>MKLSDLISRWIDVEPSKNAQIILRDRYFMKDLDGNYLETKWEDVARRVARVVATAELLNPSYKKNEKLDRIKEWEDIFFRVLKARLFIPNSPTLFNAGLGVKHDLLWKPIDQMTLEDYEEIYRSRNHLHMLSACFVVPVGDSIEEIFEAVKEYALITKVGGGVGSNFSELRPKGSFVAGTHGKASGPVSFMHVFNSAISVVKQGSRRRGALMGILNINHPDIEEFIDAKKENTGEAVLNFFNLSVGFPMDKKEILKLYEEDGELELSHPRSTIRKKVKIRELFRKIATNAWKSGDPGLAFLGEMNKYYPLYPHRKINSTNPCGEIGLSDYEACNLGSIDVAKFYNNGFVDLEALQELVQIAVRFLDNVIDVNVFPIDKITKAVKESRRLGLGIMGFADLLYKLEIP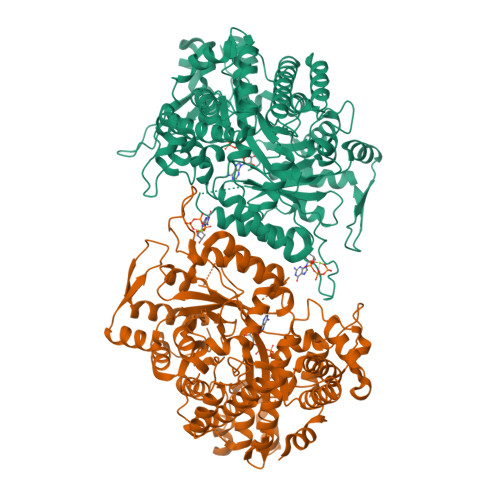YNSQEARDFAANLMAFIALHAHRTSYELGKEKGNFPLLEISRYRTEDNFVPFAMGMSNYDDEIREVMKMTKEFRRNVALLTIAPTGSISNIADTSSGLEPNFLLAYTRFVTKDDGTKEPLLYVNQVLREKLNPEILKRIEKELIEKGSLKDIPDVPEKIKKVFVVALDIDPMDHLLMQDAFQRYVDNNISKTINMPQSATVDDVLNVYLEALRTNVRGITVYRDGSLQTQVLTKALKT[2x]> GSHMAARTDNSIVVNAPFELVWDVTNDIEAWPELFSEYAEAEIL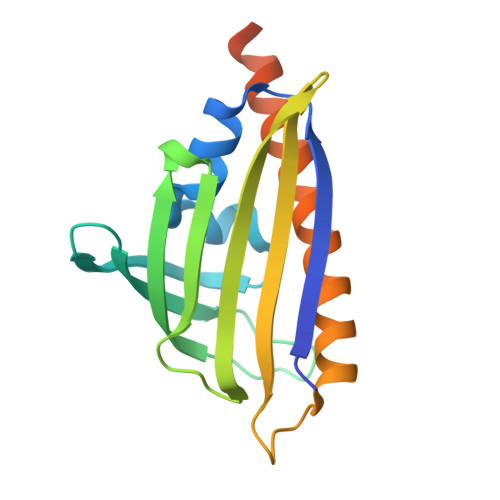RQDGDGFDFRLKTRPDANGRVWEWVSHAVPDKGSRTVRAHRVETGPFAYMNLHWTYRAVAGGTEMRWVQEFDMKPGAPFDNAHMTAHLNTTTRANMERIKKIIEDRHREGQRTPASVLPTELHAQQLLL> MAHVVILGAGTGGMPAAYEMKEALGSGHEVTLISANDYFQFVPSNPWVGVGWKERDDIAFPIRHYVERKGIHFIAQSAEQIDAEAQNITLADGNTVHYDYLMIATGPKLAFENVPGSDPHEGPVQSICTVDAAERAFAEYQALLREPGPIVIGAMAGASCFGPAYEYAMIVASDLKKRGMRDKIPSFTFITSEPYIGHLGIQGVGDSKGILTKGLKEEGIEAYTNCKVTKVEDNKMYVTQVDEKGETIKEMVLPVKFGMMIPAFKGVPAVAGVEGLCNPGGFVLVDEHQRSKKYANIFAAGIAIAIPPVETTPVPTGAPKTGYMIESMVSAA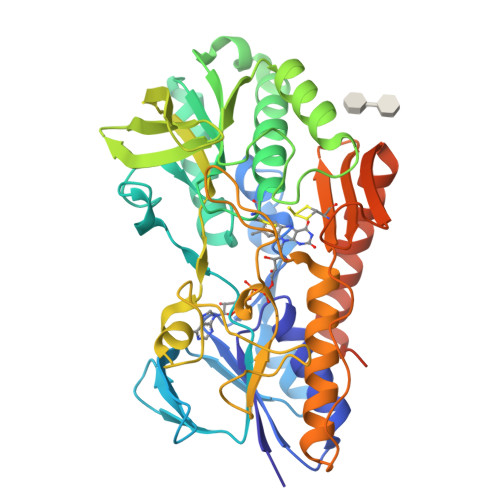VHNIKADLEGRKGEQTMGTWNAVCFADMGDRGAAFIALPQLKPRKVDVFAYGRWVHLAKVAFEKYFIRKMKMGVSEPFYEKVLFKMMGITRLKEEDTHRKAS>[2x]GGGAGCCCUGUCACCGGAUGUGCUUUCCGGUCUGAUGAGUCCGUGAGGACAAAAC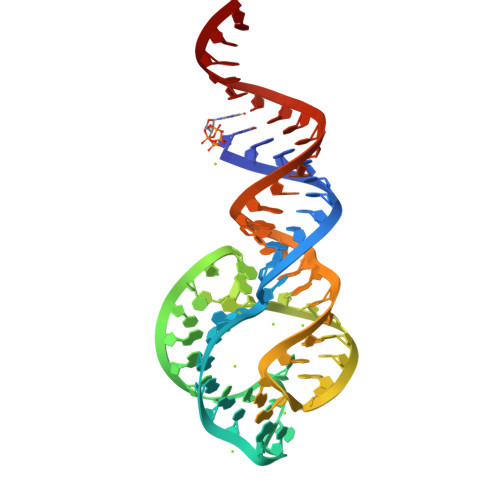AGGGCUCCCGAAUU>[3x]EPGLPPGPLENSSAKLVNDEAHPWKPLRPGDIRGPCPGLNTLASHGYLPRNGVATPAQIINAVQEGFNFDNQAAIFATYAAHLVDGNLITDLLSIGRKTRLTGPDPPPPASVGGLNEHGTFEGDASMTRGDAFFGNNHDFNETLFEQLVDYSNRFGGGKYNLTVAGELRFKRIQDSIATNPNFSFVDFRFFTAYGETTFPANLF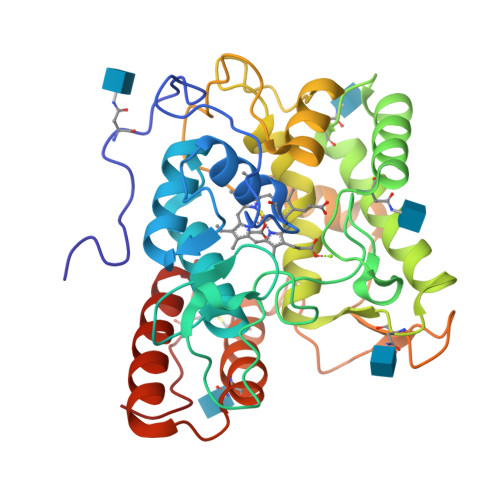VDGRRDDGQLDMDAARSFFQFSRMPDDFFRAPSPRSGTGVEVVVQAHPMQPGRNVGKINSYTVDPTSSDFSTPCLMYEKFVNITVKSLYPNPTVQLRKALNTNLDFLFQGVAAGCTQVFPYGRD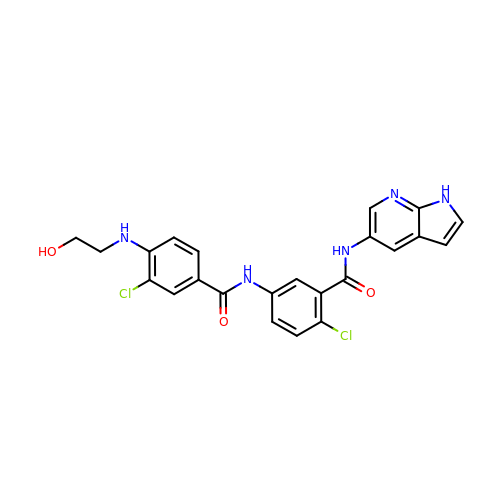2-chloro-5-{3-chloro-4-[(2-hydroxyethyl)amino]benzamido}-N-(1H-pyrrolo[2,3-b]pyridin-5-yl)benzamide | C23 H19 Cl2 N5 O3 | CFIGHGMQRALVCP-UHFFFAOYSA-N4-nitrophenyl 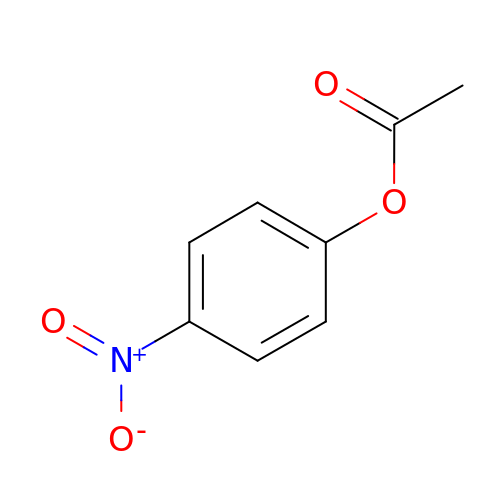acetate | C8 H7 N O4 | QAUUDNIGJSLPSX-UHFFFAOYSA-N> GSSHHHHHHSGDPASMNN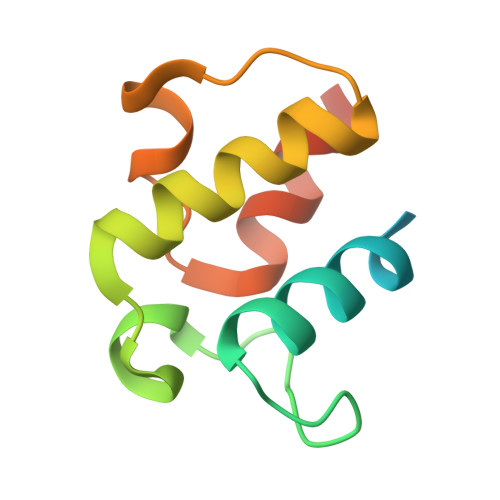HPEVKIKTILSLFLNINIDDFNMDANLADAYDMDSTELADLAKEIEKEFGISVTKSQFSHWETGRAVLDFVSSSLNDKN> MKRFARKETIYLRGEEARTLYRLEEGLVRVVELLPDGRLITLRHVLPGDYFGEEALEGKAYRYTAEAMTEAVVQGLEPRAMDHEALHRVARNLARQMRRVQAYEAH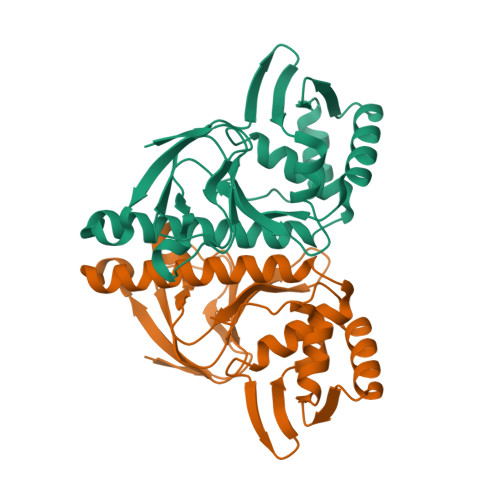LQTGELRARIARYLLFLADTPLSARDRQGIYVTVSHEEIADATASIRESVSKVLADLRREGLIATAYRRVYLLDLAALEREAGSALEAA> DVYTDHGDLYNTPVRMLVVAGAKFKEALKPWLTWKAQKGFYLDVHYTDEAEVGTTNASIKAFIHKKYNDGLAASAAPVFLALVGDTDVISGEKGKKTKKVTDLYYSAVDGDYFPEMYTFRMSASSPEELTNIIDKVLMYEKATMPDKSYLEKVLLIAGADYSWNSQVGQPTIKYGMQYYYNQEHGYTDVYNYLKAPYTGCYSHLNTGVSFANYTAHGSETAWADPLLTTSQLKALTNKDKYFLAIGNCCITAQFDYVQPCFGEVITRVKEKGAYAYIGSSPNSYWGEDYYWSVGANAVFGVQPTFEGTSMGSYDATFLEDSYNTVNSIMWAGNLAATHAGNIGNITH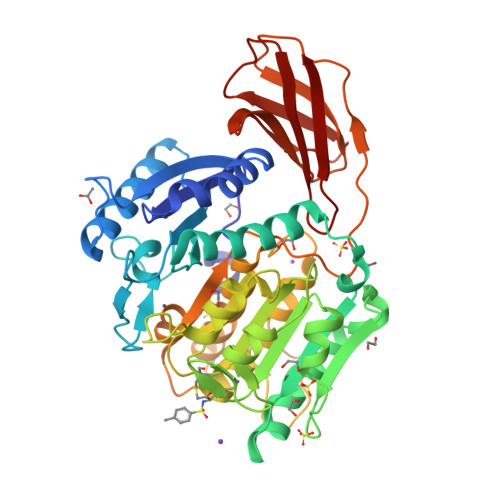IGAHYYWEAYHVLGDGSVMPYRAMPKTNTYTLPASLPQNQASYSIQASAGSYVAISKDGVLYGTGVANASGVATVSMTKQITENGNYDVVITRSNYLPVIKQIQV>MQGDPEVIEFLNEQLTAELTAINQYFLHAKLQDHKGWTKLAKYTRAESFDEMRHAEVLTDRILLLDGLPNYQRLFHVRVGQSVTEMFQADREVELEAIDRLRRGIEVMRAKHDITSANVFEAILADEEHH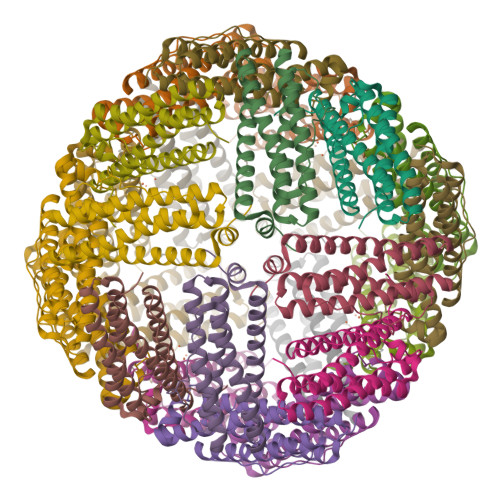IDYLETQLDLIEKLGESLYLSTVIEQTQPDPSGPGSL[6x]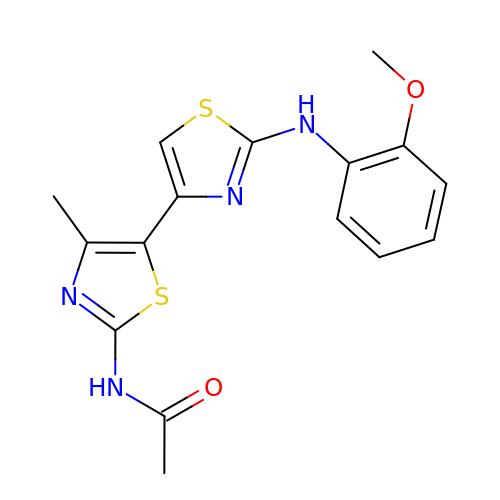~{N}-[5-[2-[(2-methoxyphenyl)amino]-1,3-thiazol-4-yl]-4-methyl-1,3-thiazol-2-yl]ethanamide | C16 H16 N4 O2 S2 | ZADCDCMLLGDCRM-UHFFFAOYSA-N In this work, we set out to find the physiological substrate of the cofactor-independent racemase (predicted DapF, FN1732) from F. nucleatum ATCC 25586, and were surprised to find that this enzyme functions as a histidine racemase (HisR). Here, we characterize this enzyme as a histidine racemase (HisR), and found that catalytic turnover is ∼10,000× faster with L-histidine than with L,L-lanthionine. The rate of HisR was not affected by buffer composition (PO4 or Tris), ions (SO42−, Mg2+, and EDTA), or the PLP inhibitor hydroxylamine; however, the enzyme activity was hindered by iodoacetamide and Hg2+, which are known inhibitors of enzymes with catalytic thiols. These results, along with a sequence alignment of HisR with other cofactor-independent racemase and epimerase enzymes, suggested that HisR operates via a two-base mechanism using cysteine residues 67 and 209. The DapF-like fold is an overall α+β structure, in which the monomer unit is composed of two structurally equivalent N-terminal and C-terminal domains.

To confirm this, we used site-directed mutagenesis to generate HisR mutants C67S and C209S. Catalytic turnover of these mutants was greatly reduced with D- and L-histidine compared to the WT enzyme, as expected. Mutation of an active site cysteine to serine is a common strategy to aid crystallization of cofactor-independent epimerases and racemases, and likely aids the process because this mutation slows catalysis and helps to keep the enzyme in the open conformation. In the asymmetric unit of C67S, there are two back-to-back dimers, while the asymmetric unit of C209S has one dimer and two monomers. Structures of C67S and C209S HisR were very similar, with a backbone r.m.s.d. of 0.493 Å by aligning α-carbons of 260 residues, and each adopt a DapF-like fold. In each structure, a sulfate (mutant C67S) or a phosphate (mutant C209S) is found in the active site directly between catalytic residues. The substrate binding pocket of HisR has an overall negatively charged surface, and does not contain any basic residues. The position of the loops above the active site spanning from residues 42 to 49 (N-terminal domain) and 197 to 206 (C-terminal domain) in HisR more closely match the conformation of the open C. glutamicum structure than the substrate-bound, closed form. Overlay of the structures of CntK and HisR showed that while these two enzymes have relatively low sequence identity (28%), their structures are overall very similar, especially within the active site. The positions of backbone atoms in DAP and 4-hydroxyproline substrates were highly conserved, and interactions with their respective epimerase enzymes were very similar.

>MDRKVQVLDFIKINPAGNITILIDNFDIYDKNIPKLSEEIMKETNLYAEQVGFIKDSHLQMMGGEFSGNASRAFASLLAFRDKDFSKQKNYNITCSGESKVLDVDVRNDGAKNKFLAKIKMPKFLSLEEINVDEYKLGLVRFSGINHFIFNIKENKETSFENIIDLVKKYLSNEEYSAFGIMFFDSDNLSMKPYVYVKEVGSGVYENSCASGTTALGYYLKKCKNLDRAKIVQPNGWLEYIIENDEMYIDGPVEIIAEGKIYIGKHHHHHH[4x]>RSPWGDELLNICMNAKHHKRVPSPEDKLYEECIPWKDNACCTLTTSWEAHLDVSPLYNFSLFHCGLLMPGCRKHFIQAICFYECSPNLGPWIQPVGSLGWEVAPSGQGERVVNVPLCQEDCEEWWEDCRMSYTCKSNWRG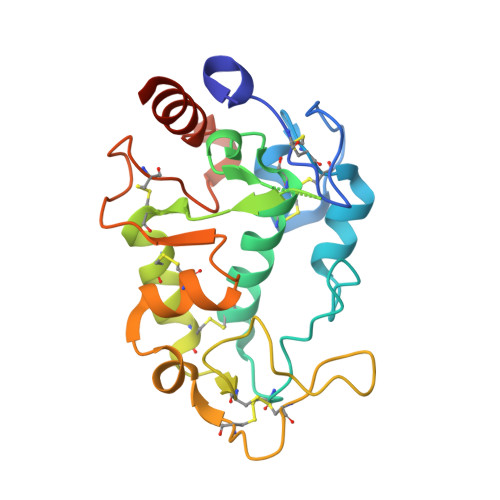GWDWSQGKNRCPKGAQCLPFSHYFPTPADLCEKTWSNSFKASPERRNSGRCLQKWFEPAQGNPNVAVARLFASEFLEVLFQ[4x]Schlafen 11 (SLFN11) is an interferon-inducible antiviral restriction factor with tRNA endoribonuclease and DNA binding functions. It is recruited to stalled replication forks in response to replication stress and inhibits replication of certain viruses such as the human immunodeficiency virus 1 (HIV-1) by modulating the tRNA pool. SLFN11 consists of an N-terminal endonuclease domain (residues 1–353), termed Slfn core domain, followed by a linker domain (residues 354–576) and a C-terminal domain with homology to superfamily I (SF I) DNA/RNA helicases (residues 577–901). SLFN11 forms a homodimer with the helicase domains adopting an autoinhibited conformation.

We found that SLFN11 binds single-strand DNA (ssDNA) with high affinity but does not bind to double-strand DNA (dsDNA). To structurally analyse the interaction between SLFN11 and ssDNA, we solved the cryo-EM structure of SLFN11 bound to 60 nt ssDNA at 3.16 Å resolution. The overall fold is similar to the structure of the apoenzyme dimer. Both protomers bind a stretch of five nucleotides via a positively charged patch between the helicase N- and C-lobes. Since the helicase domains of the two protomers are rotated by 180° relative to each other, the ssDNA strands are pointing in opposing 5’ to 3’ directions. The majority of the interactions are located along the phosphate backbone (helicase N-lobe: N633, Q634, T650, K652, T653, R656, R674; helicase C-lobe: S853, R855, R856). A single charge reversal mutation (K652D) abolishes the ssDNA binding completely. The shape of the ssDNA binding groove in SLFN11 seems to sterically prevent dsDNA binding. The sigmoid shape of the fluorescence anisotropy data suggests cooperative binding of ssDNA, consistent with the observation that both DNA binding sites are occupied in the cryo-EM structure. The opposite 5’ to 3’ direction of the two bound ssDNAs suggests that the SLFN11 dimer could simultaneously bind to both single strands at a stalled replication fork and may thereby block fork progression.

>MADYKDDDDKGTDYKDDDDKLEVLFQGPMEANQCPLVVEPSYPDLVINVGEVTLGEENRKKLQKIQRDQEKERVMRAACALLNSGGGVIRMAKKVEHPVEMGLDLEQSLRELIQSSDLQAFFETKQQGRCFYIFVKSWSSGPFPEDRSVKPRLCSLSSSLYRRSETSVRSMDSREAFCFLKTKRKPKILEEGPFHKIHKGVYQELPNSDPADPNSDPADLIFQKDYLEYGEILPFPESQLVEFKQFSTKHFQEYVKRTIPEYVPAFANTGGGYLFIGVDDKSREVLGCAKENVDPDSLRRKIEQAIYKLPCVHFCQPQRPITFTLKIVNVLKRGELYGYACMIRVNPFCCAVFSEAPNSWIVEDKYVCSLTTEKWVGMMTDTDPDLLQLSEDFECQLSLSSGPPLSRPVYSKKGLEHKKELQQLLFSVPPGYLRYTPESLWRDLISEHRGLEELINKQMQPFFRGILIFSRSWAVDLNLQEKPGVICDALLIAQNSTPILYTILREQDAEGQDYCTRTAFTLKQKLVNMGGYTGKVCVRAKVLCLSPESSAEALEAAVSPMDYPASYSLAGTQHMEALLQSLVIVLLGFRSLLSDQLGCEVLNLLTAQQYEIFSRSLRKNRELFVHGLPGSGKTIMAMKIMEKIRNVFHCEAHRILYVCENQPLRNFISDRNICRAETRKTFLRENFEHIQHIVIDEAQNFRTEDGDWYGKAKSITRRAKGGPGILWIFLDYFQTSHLDCSGLPPLSDQYPREELTRIVRNADPIAKYLQKEMQVIRSNPSFNIPTGCLEVFPEAEWSQGVQGTLRIKKYLTVEQIMTCVADTCRRFFDRGYSPKDVAVLVSTAKEVEHYKYELLKAMRKKRVVQLSDACDMLGDHIVLDSVRRFSGLERSIVFGIHPRTADPAILPNVLICLASRAKQHLYIFPWGGH[2x]> MCL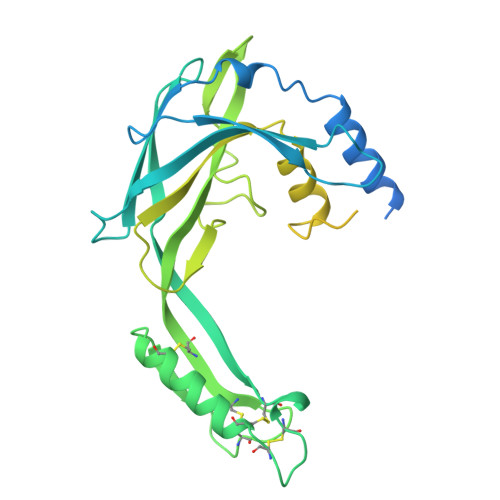FGIVDAVADFLKGVVACACCLIIGGPALIIAGSMLLNQQDLRKAFRDAVNEFNPTPMNAWTGTINDVPIAVRRESLNVKGVDGATSVFAEAVVSVSHMSSSRFQVSVNVRTVTPFNRMAPFRTIEKTSYTCSSRDCKSRLNCQCNELLNSFMNQCVASGGKFVRTPGMCVLDRTCGTCERTVYLRQLYLVVREVSNGKYAEDTNLRSAMYAFGDLDNDYQPGIPSTVTVRLYSSKDPYIALQRLTKGTNDLGLNSRTVGIVLIVLGCLFLLLEIGVCTALICYWMRRKKTSSGAPPYMAPATYGISNSGASGNAAPNFYAQPAQQTGQGYTYFQAAPPGYTYGQPPQGQPVPQGYAYGQPVSPQGQHGYTYGQAPPPLYAYGQPVSPQAPRGQVPPPL> MGHHHHHHWESKFSKEGLTFDDVLLVPAKSEVLPRDVDLSVELTKTLKLNIPV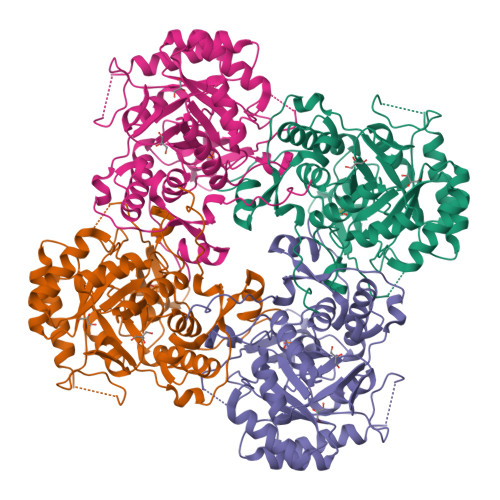ISAGMDTVTESAMAIAMARQGGLGIIHKNMSIEQQAEQVDKVKRSERGSGSEFPNSSKDIHGRLIVGAAVGVTGDTMTRVKKLVEANVDVIVIDTAHGHSQGVLNTVTKIRETYPELNIIAGNVATAEATRALIEAGADVVKVGIGPGSICTTRVVAGVGVPQITAIYDCATEARKHGKTIIADGGIKFSGDITKALAAGGHAVMLGSLLAGTSESPGETEIYQGRRFKVYRGMGSVAAMEKGSKDRYFQEENKKFVPEGIEGRTPYKGPVEETVYQLVGGLRSGMGYCGSKDLRALREEAQFIRMTGAGLRESHPHDVQITKESPNYTIS> DNSRYTHFLTQHYDAKPQGRDDRYCESIMRRRGLTSPCKDINTFI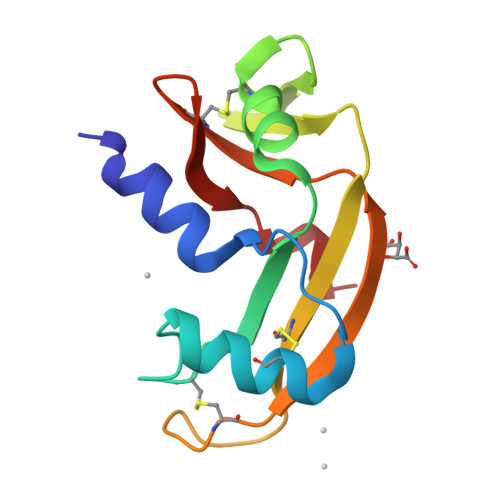HGNKRSIKAICENKNGNPHRENLRISKSSFQVTTCKLHGGSPWPPCQYRATAGFRNVVVACENGLPVHLDQSIFRR> SEKEKVEELAQRIREQLPDTELAREAQELADEARKSDDSEALKVVYLALRIVQQLPDTELAREALELAKEAVKSTDSEALKVVELALKIVQQLPDTELAKEALKLAKEAVKSTDSEALKVVELALEIVQQLPDTELAKEALELAEEAVKSTDSEALKVVKLALEIVQQLPDTELAREALELAKEAVKSTDSEALKVVYLALRIVQQLPDTELARLALELAKKAVEMTAQEVLEIARAALKAAQAFPNTELAELMLRLAEVAARVMKELERNDEEIKKSDELDDESLLEDIVELLKEIIKLWKILVEVSDVMLKLIS;> SEKEKVEELAQRIREQLPDTELAREAQELADEARKSDDSEALKVVYLALRIVQQLPDTELAREALELAKEAVKSTDSEALKVVELALKIVQQLPDTELAKEALELAKEAVKSTDSEALKVVELALEIVQQLPDTELAKEALKLAKEAVKSTDSEALKVVYLALRIVQQLPDTELAREALELAKEAVKSTDSEQLEVVRLALEIVQLAPDTRLARAALKLAKEAVKSTDQEELKKVKAILRVASEVLKLEEEAKKSQEEVERLKQEVEKASKAGLDHEGDSRIFKKIHDVVTKQIKVILRLIAVYAELVAIIG;> GSKQKEAIKVYLELLEVHSRVLKALIEQIKLFIELIMEPDEDLADKVRKSSEELKKIIKEVEKILRKVDDILEK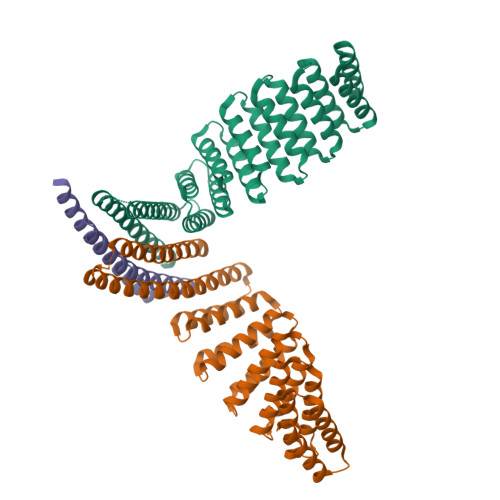VKS>MNILIFGPNGSGKGTQGNLVKDKYSLAHIESGGIFREHIGGGTELGKKAKEFIDRGDLVPDDITIPMVLETLESKGKDGWLLDGFPRNTVQAQKLFEALQEKGMKINFVIEILLPREVAKNRIMGRRICKNNPNHPNNIFIEAIKPNGDVCRVCGGALSARADDQ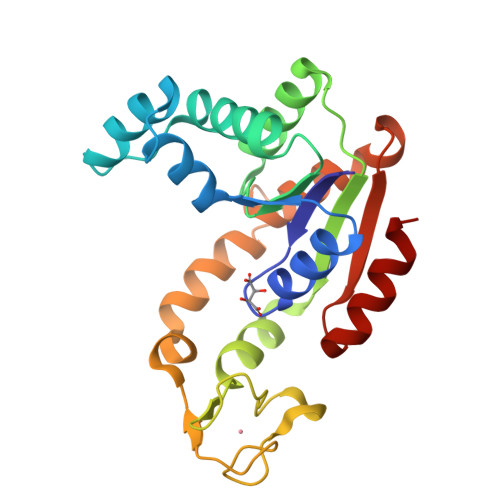DEGAINKRHDIYYNTVDGTLAAAYYYKNMAAKEGFVYIELDGEGSIDSIKDTLLAQLA[2x]>[6x]SGIVQQQNNLLRAIEAQQHLLQLTVWGTKQLQARILSGGRGG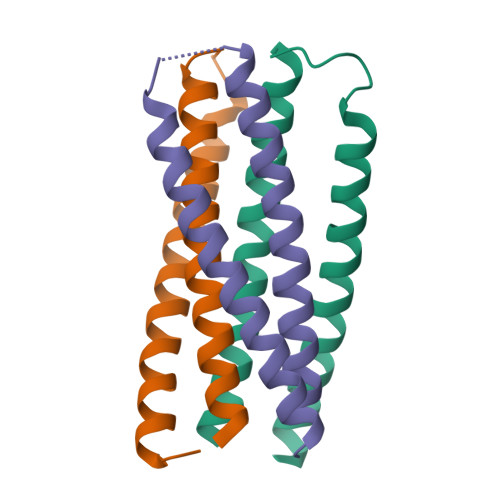WMEWDREINNYTSLIHSLIEESQNQQEKNEQELL>MEAIRKELSRSYQELNEEAEPVAIDPEEAEDEEKEQEEAASAVAPDRDSDRSSPPVRFSRTCLKNFFSVLLILVYLLLMGVAVFLVYQTITDFRDKLKHPVMSVSYKEVNMYDAPGIALYPGKARLLSCEHHWYDHIPPLKDPGQPGENTCVTQDISYIDPYTNKTMKHALIVQGPRDVRRRELVFLQFHLNETKQDFSAIDYLLFSSYEAFLKSHDQVKFMQDCE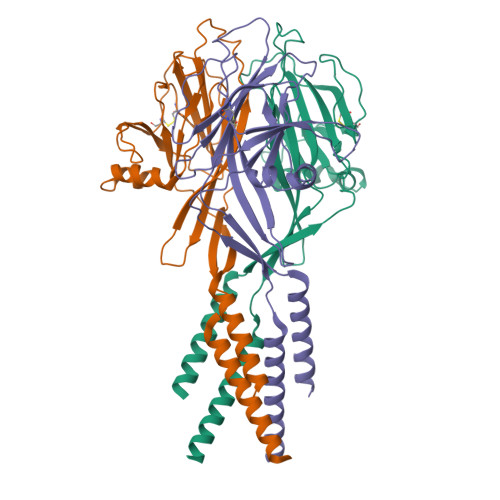SSFSSWKFSGGFRTWVKMSLVKTKEEDGSQSVEFRQETSVVNFIDRRETPDKGDQLFFVVFEWKDPYIQEIQDIITANPWSMIALLCSVFLVLFKAADFAKLSVKWMIKVRRRHLKKRARELNHIS[3x]>[4x]MNPLDLIAKRAYPYETEKRDKTYLALNENPFPFPEDLVDEVFRRLNSDALRIYYDSPDEELIEKILSYLDTDFLSKNNVSVGNGADEIIYVMMLMFDRSVFFPPTYSCYRIFAKAVGAKFLEVPLTKDLR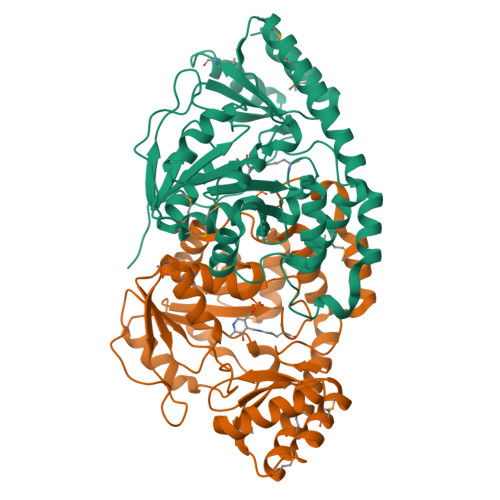IPEVNVGEGDVVFIPNPNNPTGHVFEREEIERILKTGAFVALDEAYYEFHGESYVDFLKKYENLAVIRTFSKAFSLAAQRVGYVVASEKFIDAYNRVRLPFNVSYVSQMFAKVALDHREIFEERTKFIVEERERMKSALREMGYRITDSRGNFVFVFMEKEEKERLLEHLRTKNVAVRSFREGVRITIGKREENDMILRELEVFK>[10x]MFTDTINKCAANAARIARLSANNPLGFWVSSAMAGAYVGLGIILIFTLGNLLDPSVRPLVMGATFGIALTLVIIAGSELFTGHTMFLTLGVKAGTISHGQMWAILPQTW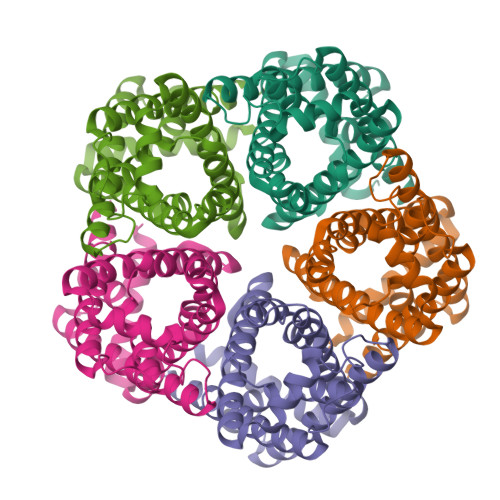LGNLVGSVFVALLYSWGGGSLLPVDTSIVHSVALAKTTAPATVLFFKGALCNWLVCLAIWMAIRTEGTAKFLAIWWCLLAFIASGYEHSVANMTLFALSWFGHHSDAYTLAGIGHNLLWVTLGNTLSGVVFMGLGYWYATPKSELEHHHHHH>[2x]NVSFPASVQLHTAVEMHHWCIPFSVDGQPAPSLRWLFNGSVLNETSFIFTEFL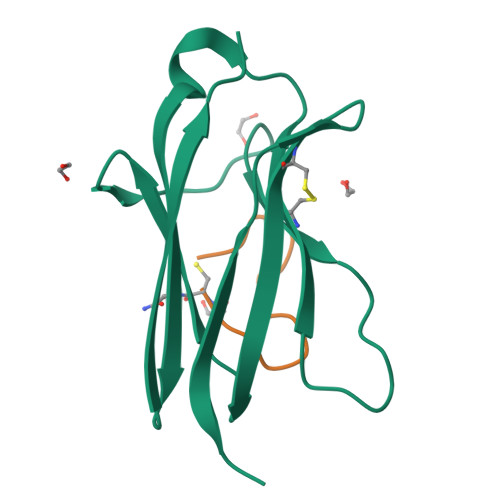EPAANETVRHGCLRLNQPTHVNNGNYTLLAANPFGQASASIMAAFMDNP;>GFFLYPHGFYGIVC[2x]> MSDKIIHLTDDSFDTDVLKADGAILVDFWAEWCGPCKMIAPILDEIADEYQGKLTVAKLNIDQNPGTAPKYGIR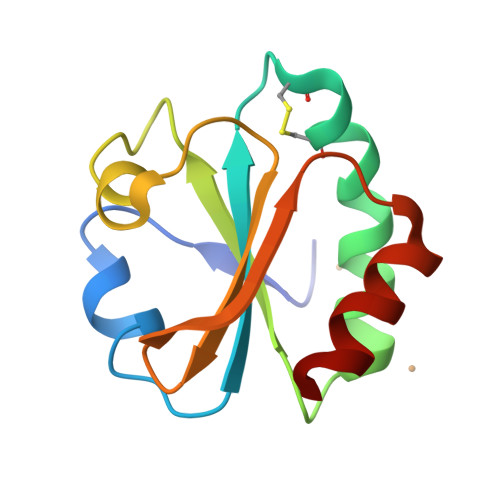GIPTLLLFKNGEVAATKVGAASKGQLKEFLDANLA>[4x]MKGTIVG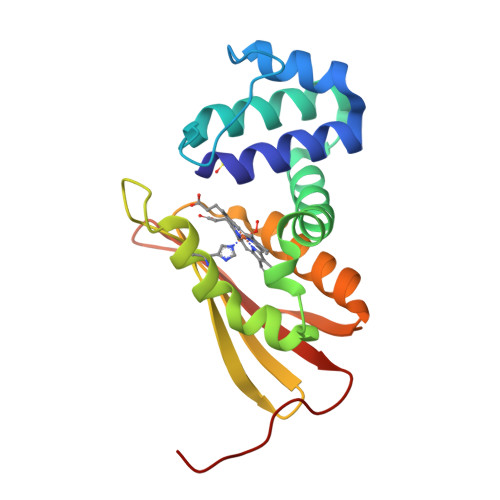TWIKTLRDLYGNDVVDESLKSVGWEPDRVITPLEDIDDDEVRRIFAKVSEKTGKNVNEIWREVGRQNIKTFSEWFPSYFAGRRLVNFLMMMDEVHLQLTKMIKGATPARLIAKPVAKDAIEMEYVSKRKMYDYFLGLIEGSSKFFKEEISVEEVERGEKDGFSRLKVRIKFKNPVFEYKKN>[2x]SPPAVPQT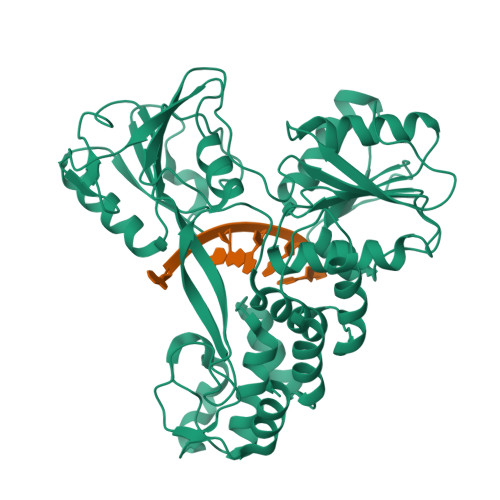FQVAHLHAPTGSGKSTKVPAAYAAQGYKVLVLNPSVAATLGFGAYMSKAHGIDPNIRTGVRTITTGAPITYSTYGKFLADGGCSGGAYDIIICDECHSTDSTTILGIGTVLDQAETAGARLVVLATATPPGSVTVPHPNIEEVALSSTGEIPFYGKAIPIETIKGGRHLIFCHSKKKCDELAAKLSGLGLNAVAYYRGLDVSVIPTSGDVIVVATDALMTGFTGDFDSVIDCNTCVTQTVDFSLDPTFTIETTTVPQDAVSRSQRRGRTGRGRMGIYRFVTPGERPSGMFDSSVLCECYDAGCAWYELTPAETSVRLRAYLNTPGLPVCQDHLEFWESVFTGLTHIDAHFLSQTKQAGDNFPYLVAYQATVCARAQAPPPSWDQMWKCLIRLKPTLHGPTPLLYRLGAVQNEVTTTHPITKYIMACMS> GPHTVAEKQDTLVPAGPAKAVLEVNDELLKAVASGDWDAYTTMVDPNVTCFEPEAAGVLAKGLAFHKFFFDNRSPNADKMKTTLHDPAVQMFGDTAIVTALRVVQFVADDGPKTTRYEETRVWVKDAAFKFGWKLVHFHRSGAHATPN

Ca2+/calmodulin-dependent protein kinase II (CaMKII) is a Ser/Thr kinase that is particularly important in neuronal signaling and cardiac function. CaMKII has a unique architecture, in which the catalytic domains are linked flexibly to a hub domain, also called the association domain, which forms a dodecameric or tetradecameric assembly (see Figure 1A for a description of the domains of CaMKII). We reported recently that the activation of CaMKII-α by ATP and Ca2+/CaM triggers the exchange of activated subunits between different holoenzyme assemblies. Our data are consistent with the idea that the CaM-binding element induces the hub to transition from a closed-ring form to a ring-opened lock-washer configuration, which can release or capture dimer units.

Choanoflagellates are the closest living relatives of metazoans. The choanoflagellate S. rosetta has one CaMKII gene. The quaternary assembly of the S. rosetta hub is strikingly different from that of all other hubs in that it forms a right-handed spiral, corresponding to a hexagonal P61 screw axis in the crystal lattice, instead of a closed ring. On looking at a projection down the hexagonal screw axis, the dimers are arrayed in a circle with almost the same diameter as that formed by the dodecameric forms of human CaMKII. An orthogonal view shows that the helical pitch of the assembly is such that the sixth dimer is displaced vertically by the length of a dimer, with respect to the first one. This positions the seventh dimer directly above the first one. At 48 μM, the tetramer and hexamer populations increase further, and a population of octamers now appears. These results are consistent with the open-ended spiral assembly of the S. rosetta hub, which can gain or lose dimer units without steric constraints. Despite the striking dissimilarity in quaternary structure, the interface that holds dimers together in all metazoan CaMKII hubs is very closely preserved in the S. rosetta hub, with helix D from one hub domain packed against the β-sheet of the adjacent domain. The principal structural difference between a subunit in a closed-ring hub and one in the spiral S. rosetta hub is a rotation in the outer edge of the β-sheet with respect to the inner edge of the sheet and the α-helices. The interfacial interactions between the vertical dimers of the hub are between residues on the outer edge of the β-sheet in one subunit, and residues presented by helix D in the other. These interfacial interactions are preserved in the S. rosetta hub, but a change in the curvature of the β-sheet results in a change in the orientation of helix D in each subunit.HmuTUV forms an ABC-type heme transporter system, in which HmuT, HmuU, and HmuV are the heme binding lipoprotein, permease, and ATPase, respectively. CgHmuT consists of two lobes connected with a α-helix, both of which consist of a five-stranded β-sheet and four α-helices. His141 and Tyr240 are coordinated to the heme as the axial ligands and Arg242 forms a hydrogen bond with Tyr240 in CgHmuT. As CgHmuT is a substrate (heme) binding protein that shuttles heme to the cognate ABC-type heme transporter CgHmuUV in Corynebacteria, the regulation of heme binding and release is very important for its physiological function.

The purified heme-bound proteins were crystallized, and the crystal structures of H141A-, Y240A-, and R242A-CgHmuT were determined in the holo-form at the resolution of 1.30, 1.65, and 1.30 Å, respectively. While two different orientations of heme were observed in Y240A-CgHmuT, heme was accommodated with a single orientation in H140A- and R242A-CgHmuT. Except for Tyr240, there was little difference in its structure including the conformation of His141 and Arg242 compared with wild-type. His141 was coordinated to the heme iron with 2.2 Å of bond distance. Two water molecules were present in the heme pocket, where Tyr240 is located in wild-type. The oxygen atom of proximal water molecule in Y240A-CgHmuT was superimposable to the oxygen atom of Tyr240 in wild-type when comparing two structures. The distances were 2.2 and 2.7 Å between the oxygen atom of proximal water molecule and iron, and between that and the nitrogen atom of the NH group in Arg242, respectively. These results indicate that the proximal water molecule is coordinated to the heme iron as an axial ligand with the formation of a hydrogen bond with Arg242, as is the case for Tyr240 in wild-type. Ferric Y240A-CgHmuT showed the Soret, α, and β peaks at 415, 575 and 540 nm, respectively, which was a typical electronic absorption spectrum of six-coordinate, low-spin (6cLC) heme with a histidine as one axial ligand. The 6cLS state is predominant in Y240A-CgHmuT, which will be caused by the hydrogen bonding interaction between the heme-bound water and Arg242.

> MASWDSPTASSNGDLIEEIQASSTSTDPRTFTGLSIVEDIGDVVPVTDNASPALPVSLTDADGNDVVVEDVSRILPLDLYGTYSKTIAGLGLVDNIVGRTVSSTEPALADTEVVTTGGHTLNAEAILNLHPTLVIIDHSIGPREVIDQIRAAGVATVIMSPQRSIASIGDDIRDIASVVGLPEEGEKLAERSVAEVEEASTVVDELTPEDPLKMVFLAARGTGGVFFILGDAYGGRDLIEGLGGVDMAAEKGIMDLAPANAEALAELNPDVFVMMSEGLVSTGGIDGLMERPGIAQTTAGQNQRVLALPDGQSLAFGAQTGELLLRASRELYVQGGELEHHHHHH>[3x]MDTRKNVSGAERKIWSLIRDCSGKLEGVTETSVLEVLLIVSRVLGIRKEDLFLKDLGVSPTEEKRILELVEKRASGYPLHYILGEKEFMGLSFLVEEGVFVPRPETEELVELALELIRKYGIKTVADIGTGSGAIGVSVAKFSDAIVFATDVSSKAVEIARKNAERHGVSDRFFVRKGEFLEPFKEKFASIEMILSNPPYVKSS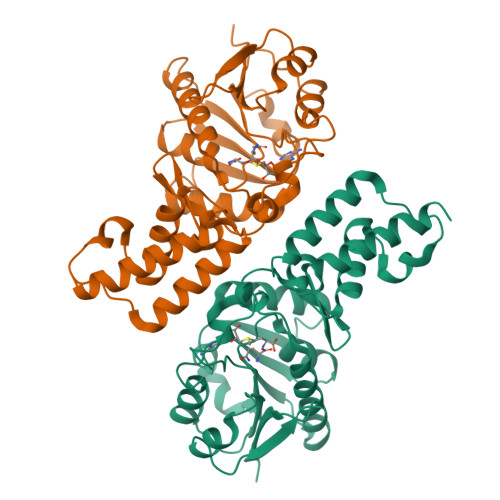AHLPKDVLFEPPEALFGGEDGLDFYREFFGRYDTSGKIVLMEIGEDQVEELKKIVSDTVFLKDSAGKYRFLLLNRRSS4'-PHOSPHOPANTETHEINE | C11 H23 N2 O7 P S | 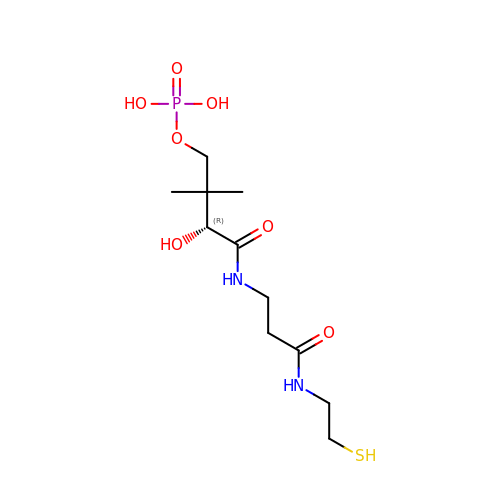JDMUPRLRUUMCTL-VIFPVBQESA-N> MSNISRQAYADMFGPTVGDKVRLADTELWIEVEDDLTTYGEEVKFGGGKVIRDGMGQGQMLAADCVDLVLTNALIVD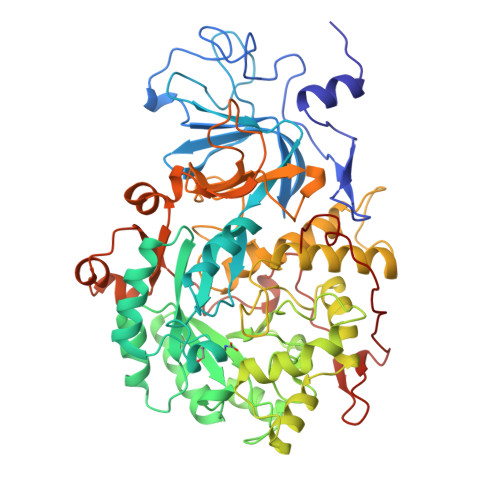HWGIVKADIGVKDGRIFAIGKAGNPDIQPNVTIPIGAATEVIAAEGKIVTAGGIDTHIHWICPQQAEEALVSGVTTMVGGGTGPAAGTHATTCTPGPWYISRMLQAADSLPVNIGLLGKGNVSQPDALREQVAAGVIGLKIHEDWGATPAAIDCALTVADEMDIQVALHSDTLNESGFVEDTLAAIGGRTIHTFHTEGAGGGHAPDIITACAHPNILPSSTNPTLPYTLNTIDEHLDMLMVAHHLDPDIAEDVAFAESRIRRETIAAEDVLHDLGAFSLTSSDSQAMGRVGEVILRTWQVAHRMKVQRGALAEETGDNDNFRVKRYIAKYTINPALTHGIAHEVGSIEVGKLADLVVWSPAFFGVKPATVIKGGMIAIAPMGDINASIPTPQPVHYRPMFGALGSARHHCRLTFLSQAAAANGVAERLNLRSAIAVVKGCRTVQKADMVHNSLQPNITVDAQTYEVRVDGELITSEPADVLPMAQRYFLF> MNPETMNENGKSLKILFTALFGPGHLNACLGIGSLLRKRGHQIYFAHFPRHRATIEKHGFLFISLLDYAEPEFPIVDMLPDIGIIAKFAFERMHKLTPLELFRHASGKHTFAGMVNGSKGENYAMMKIVKEYKPDVCLADYLFNMPWMFTVDCPVIPVKSVNPIELYNGPPALTGCSIHDPPSVREEIEQLARKSELELESELEKLFAHFNVPLVSYNYAQQLGIYIYPGPLDYKELGSPKENWVRLDSSIRSTEISNFELPEKLKDKPGKLIYVSMGSLASAVTELLTMILTPLANSPHRFIVSTGPNGDSIKLYDNMWGDKFINQVALLPKVDLFITHGGSNSLIEGLTAGKPLIAIPQFGDQLDNAQRIADLGLGVRLNLHEFSGEKLLKAIE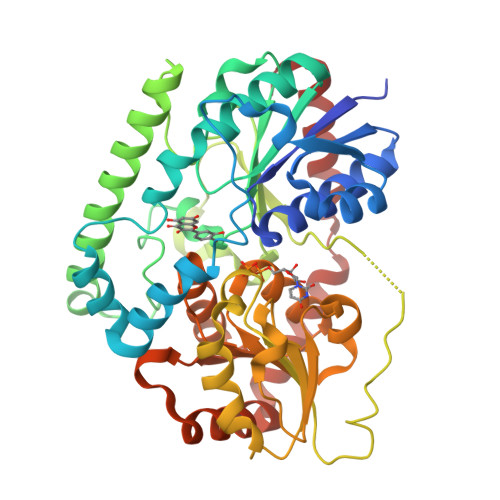DVLNDEKINANVARVSEELKKSDSKDKVISLIEKLARDKKL>MGSSHHHHHSSGENLYFQGHMSFDLIIKNGTVILENEARVVDIAVKGGKIAAIGQDLGDAKEVMDASGLVVSPGMVDAHTHISEPGRSHWEGYETGTRAAAKGGITTMIEMPLNQLPATVDRASIELKFDAAKGKLTIDAAQLGGLVSYNIDRLHELDEVGVVGFKCFVATCGDRGIDNDFRDVNDWQFFKGAQKLGELGQPVLVHCENALICDELGEEAKREGRVTAHDYVASRPVFTEVEAIRRVLYLAKVAGCRLHVCHVSSPEGVEEVTRARQEGQDITCESCPHYFVLDTDQFEEIGTLAKCSPPIRDLENQKGMWEKLFNGEIDCLVSDHSPCPPEMKAGNIMKAWGGIAGLQSCMDVMFDEAVQ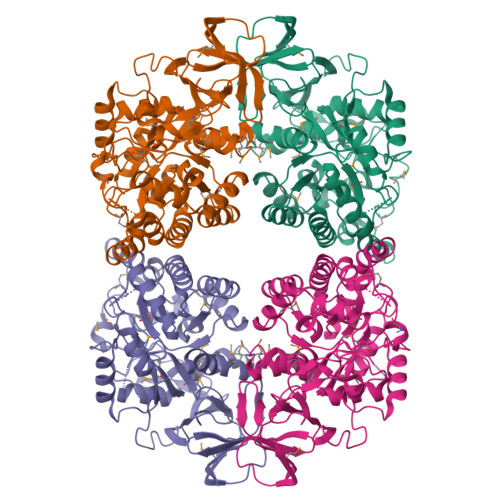KRGMSLPMFGKLMATNAADIFGLQQKGRIAPGKDADFVFIQPNSSYVLTNDDLEYRHKVSPYVGRTIGARITKTILRGDVIYDIEQGFPVAPKGQFILKHQQ[4x]>TKDNLTGDIVIIGAGAAGSLLAHYLARFSNMKIILLEAGHSHFNDPVVTDPMGFFGKYNPPNENISMSQNPSYSWQGAQEPNTGAYGNRPIIAHGMGFGGSTMINRLNLVVGGRTVFDNDWPVGWKYDDVKNYFRRVLVDINPVRDNTKASITSVALDALRIIAEQQIASGE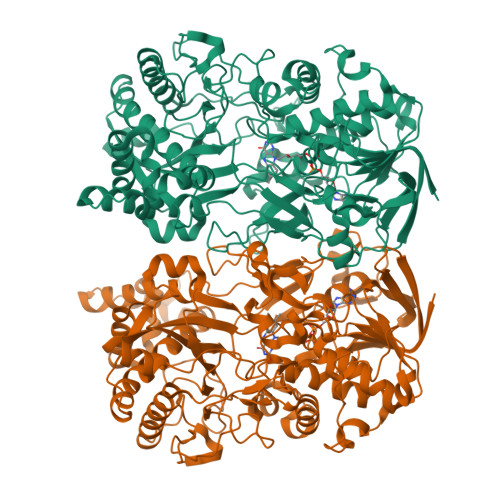PVDFLLNKATGNVPNVEKTTPDAVPLNLNDYEGVNSVVAFSSFYMGVNQLSDGNYIRKYAGNTYLNRNYVDENGRGIGKFSGLRVVSDAVVDRIIFKGNRAVGVNYIDREGIMHYVKVNKEVVVTSGAFYTPTILQRSGIGDFTYLSSIGVKNLVYNNPLVGTGLKNHYSPVTITRVHGEPSEVSRFLSNMAANPTNMGFKGLAELGFHRLDPNKPANANTVTYRKYQLMMTAGVGIPAEQQYLSGLSPSSNNLFTLIADDIRFAPEGYIKIGTPNIPRDVPKIFFNTFVTYTPTSAPADQQWPIAQKTLAPLISALLGYDIIYQTLMSMNQTARDSGFQVSLEMVYPLNDLIYKLHNGLATYGANWWHYFVPTLVGDDTPAGREFADTLSKLSYYPRVGAHLDSHQGCSCSIGRTVDSNLKVIGTQNVRVADLSAAAFPPGGNTWATASMIGARAVDLILGFPYLRDLPVNDVPILNVN[8x]> VH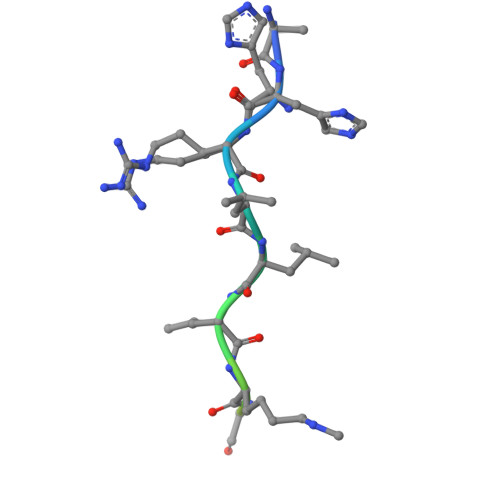RLLRKGNYAERVGA[4-(4-HYDROXY-3-ISOPROPYL-PHENOXY)-3,5-DIMETHYL-PHENYL]-6-AZAURACIL | 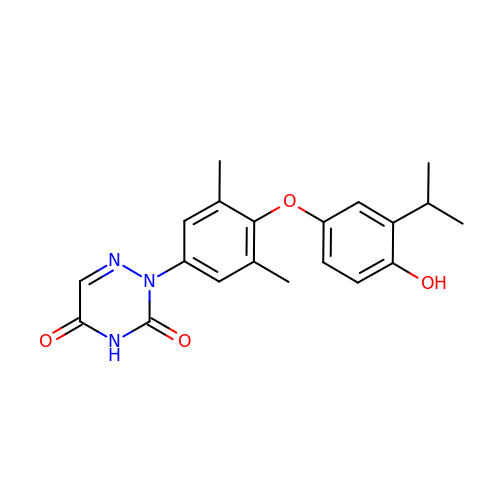C20 H21 N3 O4 | RXQAVKWRCZYGMV-UHFFFAOYSA-N>MNVIAILNHMGVYFKEEPIRELHRALERLNFQIVYPNDRDDLLKLIENNARLCGVIFDWDKYNLELCEEISKMNENLPLYAFANTYSTLDVSLNDLRLQISFFEYALGAAEDIANKIKQTTDEYINTILPPLTKALFKYVREGKYTFCTPGHMGGTAFQKSPVGSLFYDFFGPNTMKSDISISVSELGSLLDHSGPHKEAEQYIARVFNADRSYMVTNGTSTANKIVGMYSAPAGSTILIDRNCHKSLTHLMMMSDVTPIYFRPTR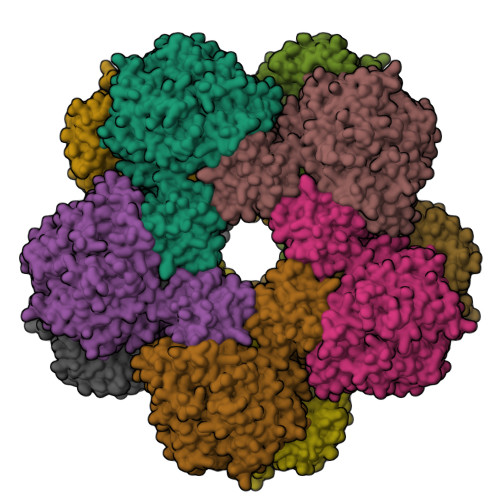NAYGILGGIPQSEFQHATIAKRVKETPNATWPVHAVITNSTYDGLLYNTDFIKKTLDVKSIHFDSAWVPYTNFSPIYEGKCGMSGGRVEGKVIYETQSTHKLLAAFSQASMIHVKGDVNEETFNEAYMMHTTTSPHYGIVASTETAAAMMKGNAGKRLINGSIERAIKFRKEIKRLRTESDGWFFDVWQPDHIDTTECWPLRSDSTWHGFKNIDNEHMYLDPIKVTLLTPGMEKDGTMSDFGIPASIVAKYLDEHGIVVEKTGPYNLLFLFSIGIDKTKALSLLRALTDFKRAFDLNLRVKNMLPSLYREDPEFYENMRIQELAQNIHKLIVHHNLPDLMYRAFEVLPTMVMTPYAAFQKELHGMTEEVYLDEMVGRINANMILPYPPGVPLVMPGEMITEESRPVLEFLQMLCEIGAHYPGFETDIHGAYRQADGRYTVKVLKEESKK[5x]>[2x]AQLCDQYA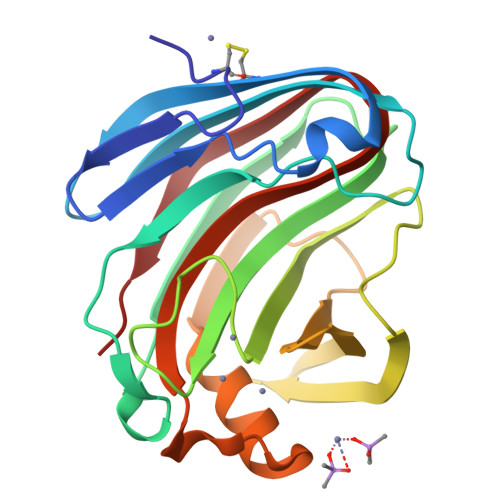TYTGGVYTINNNLWGKDAGSGSQCTTVNSASSAGTSWSTKWNWSGGENSVKSYANSGLTFNKKLVSQISQIPTTARWSYDNTGIRADVAYDLFTAADINHVTWSGDYELMIWLARYGGVQPIGSQIATATVDGQTWELWYGANGSQKTYSFVAPTPITSFQGDVNDFFKYLTQNHGFPASSQYLITLQFGTEPFTGGPATLSVSNWSASVQ> MKQYLELMQKVLDEGTQKNDRTGTGTLSIFGHQMRFNLQDGFPLVTTKRCHLRSIIHELLWFLQGDTNIAYLHENNVTIWDEWADENGDLGPVYGKQWRAWPTPDGRHIDQITTVLNQLKNDPDSERIIVSAWNVGELDKMALAPCHAFFQFYVADGKLSCQLYQRSCDVFLGLPFNIASYALLVHMMAQQCDLEVGDFVWTGGDTHLYSNHMDQTHLQLSREPRPLPKLIIKRKPESIFDYRFEDFEIEGYDPHPGIKAPV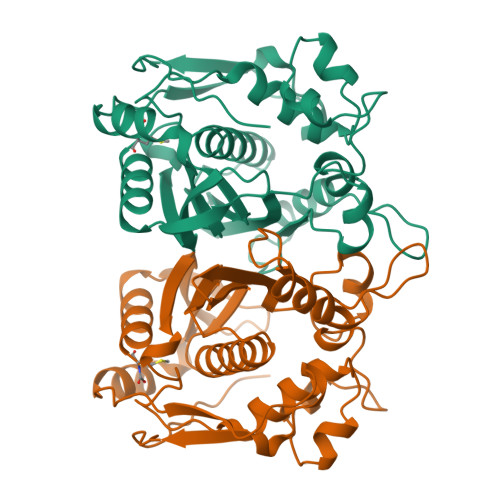AI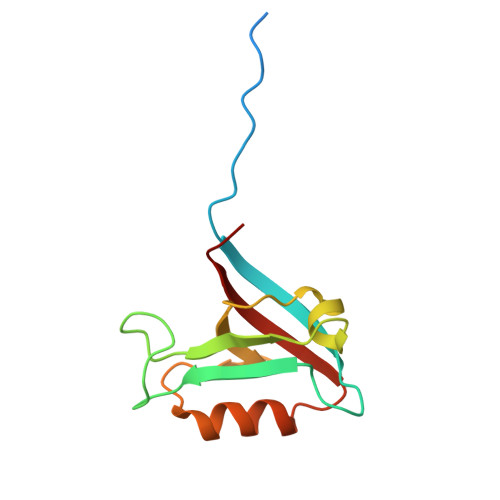> SAPSVKGVSFDQANNLLIEPARIEEEELTLTILRQTGGLGISIAGGKGSTPYKGDDEGIFISRVSEEGPAARAGVRVGDKLLEVNGVALQGAEHHEAVEALRGAGTAVQMRVWRERM>[3x]MKNEKLAKGEMNLNALFIGDKAENGQLYKDLLIDLVDEHLGWRQNYMPQDMPVISSQERTSKSYEKTVNHMKDVLNEISSRMRTHSVPWHTAGRYWGHMNSETLMPSLLAYNFAMLWNGNNVAYESSPATSQMEEEVGHEFAHLMSYKNGWGHIVADGSLANLEGLWYARNIKSLPFAMKEVKPELVAGKSDWELLNMPTKEIMDLLESAEDEIDEIKAHSARSGKHLQAIGKWLVPQTKHYSWLKAADIIGIGLDQVIPVPVDHNYRMDINELEKIVRGLAEEQIPVLGVVGVVGSTEEGAVDSIDKIIALRDELMKDGIYYYVHVDAAYGGYGRAIFLDEDNNFIPYEDLQD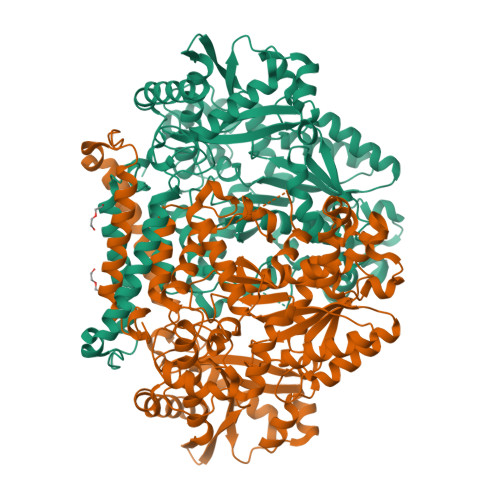VHEEYGVFKEKKEHISREVYDAYKAIELAESVTIDPHKMGYIPYSAGGIVIQDIRMRDVISYFATYVFEKGADIPALLGAYILEGSKAGATAASVWAAHHVLPLNVAGYGKLIGASIEGSHHFYNFLNDLTFKVGDKEIEVHTLTHPDFNMVDYVFKEKGNDDLVAMNKLNHDVYDYASYVKGNIYNNEFITSHTDFAIPDYGNSPLKFVNSLGFSDEEWNRAGKVTVLRAAVMTPYMNDKEEFDVYAPKIQAALQEKLEQIYDVK>XGEIAQALKEIAKALKEIAWACKEIAQA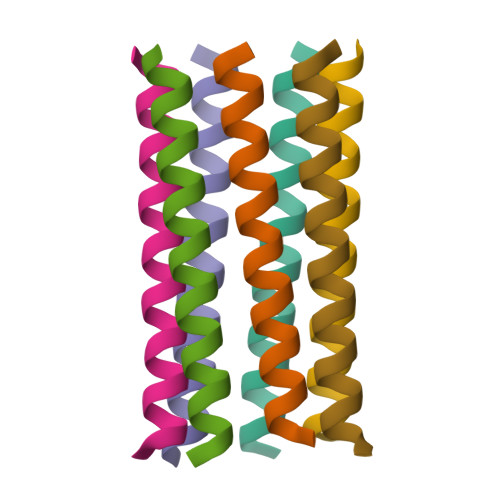LKG[7x]>[6x]MALISQSIKNLKGGISQQPDILRYPDQGSRQVNGWSSETEGLQKRPPLVFLNTLGDNGALGQAPYIHLINRDEHEQYYAVFTGSGIRVFDLSGNEKQVRYPNGSNYIKTANPRNDLRMVTVADYTFIVNRNVVAQKNTKSVNLPNYNPNQDGLINVRGGQYGRELIVHINGKDVAKYKIPDGSQPEHVNNTDAQWLAEELAKQMRTNLSDWTVNVGQGFIHVTAPSGQQIDSFTTKDGYADQLINPVTHYAQSFSKLPPNAPNGYMVKIVGDASKSADQYYVRYDAERKVWTETLGWNTEDQVLWETMPHALVRAADGNFDFKWLEWSPKSCGDVDTNPWPSFVGSSINDVFFFRNRLGFLSGENIILSRTAKYFNFYPASIANLSDDDPIDVAVSTNRIAILKYAVPFSEELLIWSDEAQFVLTASGTLTSKSVELNLTT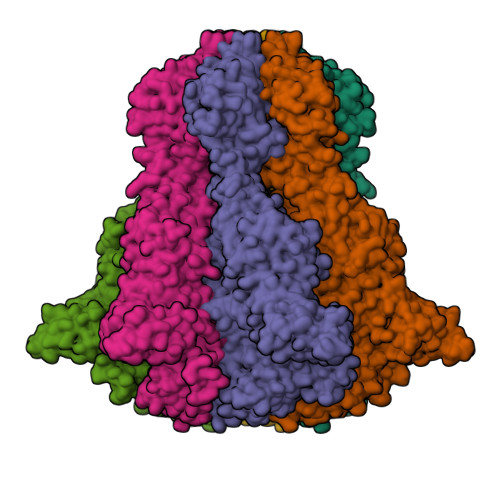QFDVQDRARPFGIGRNVYFASPRSSFTSIHRYYAVQDVSSVKNAEDITSHVPNYIPNGVFSICGSGTENFCSVLSHGDPSKIFMYKFLYLNEELRQQSWSHWDFGENVQVLACQSISSDMYVILRNEFNTFLARISFTKNAIDLQGEPYRAFMDMKIRYTIPSGTYNDDTFTTSIHIPTIYGANFGRGKITVLEPDGKITVFEQPTAGWNSDPWLRLSGNLEGRMVYIGFNINFVYEFSKFLIKQTADDGSTSTEDIGRLQLRRAWVNYENSGTFDIYVENQSSNWKYTMAGARLGSNTLRAGRLNLGTGQYRFPVVGNAKFNTVYILSDETTPLNIIGCGWEGNYLRRSSGI> RVCPKILMECKKDSDCLA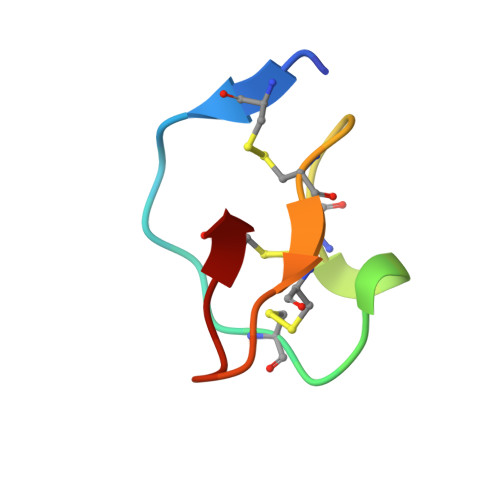ECICLEHGYCG>[3x]MDNKLGLNKMNKTLIALAVSAAAVATGAYADGINQSGDKAGSTVYSAKGTSLEVGGRAEARLSLKDGKAQDNSRVRLNFLGKAEINDSLYGVGFYEGEFTTNDQGKNASNNSLDNRYTYAGIGGTYGEVTYGKNDGALGVITDFTDIMSYHGNTAAEKIAVAD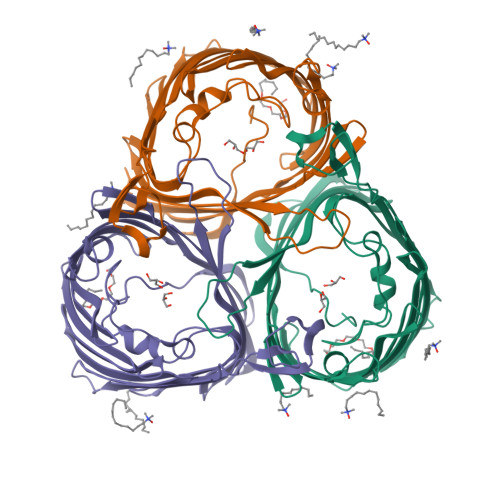RVDNMLAYKGQFGDLGVKASYRFADRNAVDAMGNVVTETNAAKYSDNGEDGYSLSAIYTFGDTGFNVGAGYADQDDQNEYMLAASYRMENLYFAGLFTDGELAKDVDYTGYELAAGYKLGQAAFTATYNNAETAKETSADNFAIDATYYFKPNFRSYISYQFNLLDSDKVGKVASEDELAIGLRYDFHHHHHH> MTQEQANQSETKPAFDFKPFAPGYAEDPFPAIERLREATPIFYWDEGRSWVLTRYHDVSAVFRDERFAVSREEWESSAEYSSAIPELSDMKKYGLFGLPPEDHARVRKLVNPSFTSRAIDLLRAEIQRTVDQLLDARSGQEEFDVVRDYAEGIPMRAISALLKVPAECDEKFRRFGSATARALGVGLVPRVDEETKTLVASVTEGLALLHGVLDERRRNPLENDVLTMLLQAEADGSRLSTKELVALVGAIIAAGTDTTIYLIAFAVLNLLRSPEALELVKAEPGLMRNALDEVLRFDNILRIGTVRFARQDLEYCGASIKKGEMVFLLIPSALRDGTVFSRPDVFDVRRDTSASLAYGRGPHVCPGVSLARLEAEIAVGTIFRRFPEMKLKETPVFGYHPAFRNIESL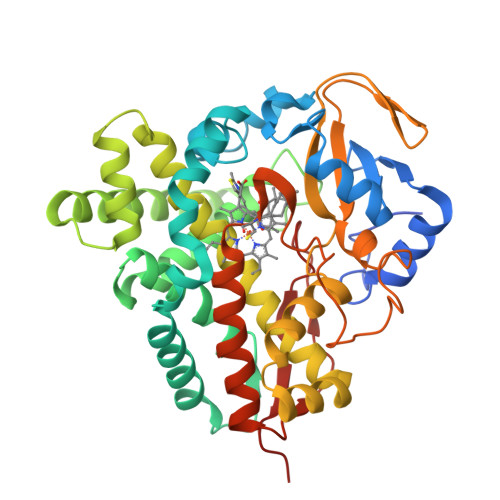NVILKPSKAG In bacteria, however, a different strategy employing a class of enzyme known as polysaccharide lyases (PL) is deployed. PLs selectively target glycans composed of uronic acids with a C4 hydroxyl group linked to the preceding sugar in the glycan chain. This enables PLs to operate through a β-elimination mechanism that relies on proton abstraction from the C5 carbon of the uronic acid sugar ring, resulting in double bond formation between C4 and C5 and elimination of the preceding sugar. The three characterized PL33_1 enzymes were all from Bacteroides species inhabiting the human colon: BT4410 (BtPL33HA) and BcellWH2_04512 (BcPL33HA) are hyaluronidases from Bacteroides thetaiotaomicron VPI-5482 (B. theta) and Bacteroides cellulosilyticus WH2 (B. cell), respectively, while HMPREF1181_01744 (BsPL33Heparosan) is a heparosanase from Bacteroides stercoris CC31F (B. stercoris). The enzymes are 68% identical and contain a larger N-terminal α-helical (α/α)6 toroid domain (residues 21 to 401; BtPL33HA numbering used throughout this section unless specified) and a smaller β-sheet C-terminal domain (residues 402 to 635).

Crystal structures of BtPL33HA and BcPL33HA reveal a two-domain structure. The C-terminal domain possesses an extended loop region between β-strands 5 and 6 (Leu455-Leu484: BtPL33HA, and Ile464-Leu493: BcPL33HA), forming an octahedral Zn2+ coordination site [supported by anomalous X-ray diffraction data], along with the loop region between α-helices 12 and 13 from the N-terminal domain. The two domains oppose each other in such a way that a deep, open-ended cleft is formed resembling an active site that would be compatible with an endo-processive mode of action of BtPL33HA and BcPL33HA. Analysis using the Consurf server, which maps residue conservation from a sequence alignment to the structure, demonstrated a high level of amino acid conservation within the cleft, consistent with it housing the active site residues. Analysis of the five enzymes via SEC-coupled light scattering and SAXS indicated that the three PL33_1 enzymes BtPL33HA, BcPL33HA, and BsPL33Heparosan are dimeric, while the PL33_2 enzymes ObPL33CS and ObPL33Gellan are monomeric. SAXS data indicate that the dimeric enzymes all bind as head-to-head homodimers, generating elongated envelopes. This is consistent with PISA analysis of the crystal structures of BtPL33HA and BcPL33HA which predicted a buried surface area of ~1,388 Å2 and 1,006 Å2, and a complex significance score of 0.207 and 0.290, respectively. For all five of the analyzed enzymes, AF2-generated models display a closed tunnel-like topography housing the +2 and +1 subsites. The phenol of Y470 moves within 5 to 6 Å of the +1 GlcA and N-acetyl of the −1 GlcNAc, while F475 moves within 5 Å of the +2 GlcNAc, forming the tunnel topography. This differs significantly from the wide-open cleft observed in the crystal structures of both BtPL33HA and BcPL33HA.

> MGSSHHHHHHSSGPQQGLRYTERNLLQKAAGSEEQLKEALVMNQKWVPYPAYNDRAGWNELLGTNKESLIRAGEKMLNYEWKVIRATDYLEYERSGERNIMQNPYEANRKAINALMLAELAEGKGRFIDQLINGAFYSCEMTSWVLSAHLVRQSTKRSLPDYREQVIDLGSGNFGSMLSWVYYFFHDSFDKIDPVISQRLRHTLQERILDPYMNNDREWWMAFQWKPGMIINNWNPWCNSNVLQCYLLLENDRDRLAKAVWRSMQSVDKFINFVKADGACEEGPSYWGHAAGKMYDYLQILSDGTDGKVSLFKEPMIRRMGEYISRTYVGNGWVVNFADASAKGGGDAPLIYRYGRAVGSEEMMQFAAYLLDGKRPSVPLGNDTFRSLQSILWNGELEKTTAAHTIPACTWYPETEFCYLTNKSGWFLATKGGFNNESHNHNDVGTFSLYVNTIPVLIDAGVGTYTRQTFSSERYTIWTMQSNYHNLPMINGVPQSFGQNYKATDVVCQPKKRFFSANIATAYPKEAEVNSWTRAYSLGDKQLTITDNFSLKSAKESNQVNFLTWGKVDISVPGKVTIDVQGQKVTLEYPGEFTATVETINLPDTRLSNVWGTEIYRIALKDKDARLTGKYKFVIK[6-hydroxy-3-(3-methylbenzyl)-1H-indazol-5-yl][(3S)-3-hydroxypyrrolidin-1-yl]methanone | C20 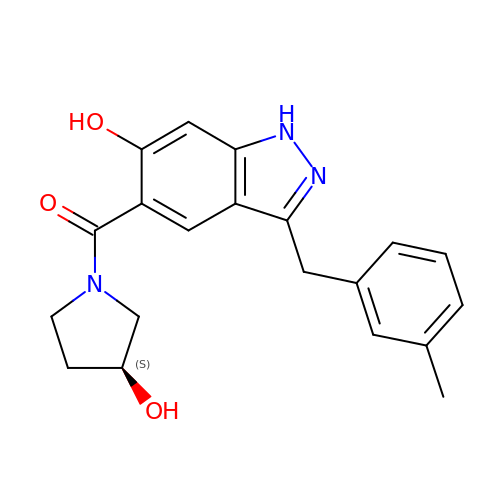H21 N3 O3 | MTAMTSBOGRBXGX-AWEZNQCLSA-N> TTPLVHVASVEKGRSYEDFQKVYNAIALKLREDDEYDNYIGYGPVLVRLAWHTSGTWDKHDNTGGSYGGTYRFKKEFNDPSNAGLQNGFKFLEPIHKEFPWISSGDLFSLGGVTAVQEMQGPKIPWRCGRVDTPEDTTPDNGRLPDA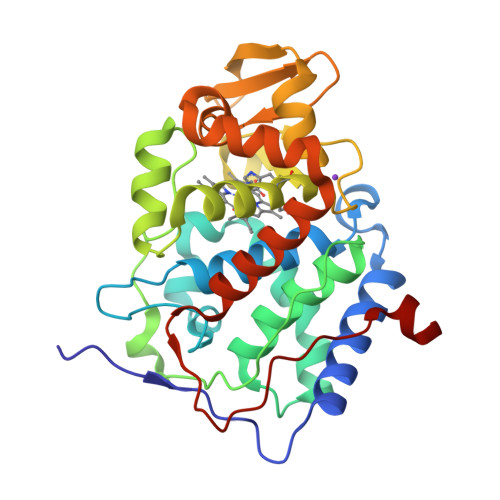DKDADYVRTFFQRLNMNDREVVALMGAHTLGKTHLKNSGYEGPWTANNNVFDNSFYLNLLNEDWKLEKNDANNEQWDSKSGYMMLPTDYSLIQDPKYLSIVKEYANDQDKFFKDFSKAFEKLLENGITFPKDAPSPFIFKTLEEQGL> MGFVRQIQLLLWKNWTLRKRQKIRFVVELVWPLSLFLVLIWLRNANPLYSHHECHFPNKAMPSAGMLPWLQGIFCNVNNPCFQSPTPGESPGIVSNYNNSILARVYRDFQELLMNAPESQHLGRIWTELHILSQFMDTLRTHPERIAGRGIRIRDILKDEETLTLFLIKNIGLSDSVVYLLINSQVRPEQFAHGVPDLALKDIACSEALLERFIIFSQRRGAKTVRYALCSLSQGTLQWIEDTLYANVDFFKLFRVLPTLLDSRSQGINLRSWGGILSDMSPRIQEFIHRPSMQDLLWVTRPLMQNGGPETFTKLMGILSDLLCGYPEGGGSRVLSFNWYEDNNYKAFLGIDSTRKDPIYSYDRRTTSFCNALIQSLESNPLTKIAWRAAKPLLMGKILYTPDSPAARRILKNANSTFEELEHVRKLVKAWEEVGPQIWYFFDNSTQMNMIRDTLGNPTVKDFLNRQLGEEGITAEAILNFLYKGPRESQADDMANFDWRDIFNITDRTLRLVNQYLECLVLDKFESYNDETQLTQRALSLLEENMFWAGVVFPDMYPWTSSLPPHVKYKIRMDIDVVEKTNKIKDRYWDSGPRADPVEDFRYIWGGFAYLQDMVEQGITRSQVQAEAPVGIYLQQMPYPCFVDDSFMIILNRCFPIFMVLAWIYSVSMTVKSIVLEKELRLKETLKNQGVSNAVIWCTWFLDSFSIMSMSIFLLTIFIMHGRILHYSDPFILFLFLLAFSTATIMLCFLLSTFFSKASLAAACSGVIYFTLYLPHILCFAWQDRMTAELKKAVSLLSPVAFGFGTEYLVRFEEQGLGLQWSNIGNSPTEGDEFSFLLSMQMMLLDAAVYGLLAWYLDQVFPGDYGTPLPWYFLLQESYWLGGEGCSTREERALEKTEPLTEETEDPEHPEGIHDSFFEREHPGWVPGVCVKNLVKIFEPCGRPAVDRLNITFYENQITAFLGHNGAGKTTTLSILTGLLPPTSGTVLVGGRDIETSLDAVRQSLGMCPQHNILFHHLTVAEHMLFYAQLKGKSQEEAQLEMEAMLEDTGLHHKRNEEAQDLSGGMQRKLSVAIAFVGDAKVVILDEPTSGVDPYSRRSIWDLLLKYRSGRTIIMSTHHMDEADLLGDRIAIIAQGRLYCSGTPLFLKNCFGTGLYLTLVRKMKNIQSQRKGSEGTCSCSSKGFSTTCPAHVDDLTPEQVLDGDVNELMDVVLHHVPEAKLVECIGQELIFLLPNKNFKHRAYASLFRELEETLADLGLSSFGISDTPLEEIFLKVTEDSDSGPLFAGGAQQKRENVNPRHPCLGPREKAGQTPQDSNVCSPGAPAAHPEGQPPPEPECPGPQLNTGTQLVLQHVQALLVKRFQHTIRSHKDFLAQIVLPATFVFLALMLSIVIPPFGEYPALTLHPWIYGQQYTFFSMDEPGSEQFTVLADVLLNKPGFGNRCLKEGWLPEYPCGNSTPWKTPSVSPNITQLFQKQKWTQVNPSPSCRCSTREKLTMLPECPEGAGGLPPPQRTQRSTEILQDLTDRNISDFLVKTYPALIRSSLKSKFWVNEQRYGGISIGGKLPVVPITGEALVGFLSDLGRIMNVSGGPITREASKEIPDFLKHLETEDNIKVWFNNKGWHALVSFLNVAHNAILRASLPKDRSPEEYGITVISQPLNLTKEQLSEITVLTTSVDAVVAICVIFSMSFVPASFVLYLIQERVNKSKHLQFISGVSPTTYWVTNFLWDIMNYSVSAGLVVGIFIGFQKKAYTSPENLPALVALLLLYGWAVIPMMYPASFLFDVPSTAYVALSCANLFIGINSSAITFILELFENNRTLLRFNAVLRKLLIVFPHFCLGRGLIDLALSQAVTDVYARFGEEHSANPFHWDLIGKNLFAMVVEGVVYFLLTLLVQRHFFLSQWIAEPTKEPIVDEDDDVAEERQRIITGGNKTDILRLHELTKIYPGTSSPAVDRLCVGVRPGECFGLLGVNGAGKTTTFKMLTGDTTVTSGDATVAGKSILTNISEVHQNMGYCPQFDAIDELLTGREHLYLYARLRGVPAEEIEKVANWSIKSLGLTVYADCLAGTYSGGNKRKLSTAIALIGCPPLVLLDEPTTGMDPQARRMLWNVIVSIIREGRAVVLTSHSMEECEALCTRLAIMVKGAFRCMGTIQHLKSKFGDGYIVTMKIKSPKDDLLPDLNPVEQFFQGNFPGSVQRERHYNMLQFQVSSSSLARIFQLLLSHKDSLLIEEYSVTQTTLDQVFVNFAKQQTESHDLPLHPRAAGASRQAQD

ABCA4 is an ATP-binding cassette (ABC) transporter that flips N-retinylidene-phosphatidylethanolamine (N-Ret-PE) from the lumen to the cytoplasmic leaflet of photoreceptor membranes. Human ABCA4 is a 2273 amino acid full transporter organized in two nonidentical tandem halves with each half containing a transmembrane domain (TMD) consisting of six membrane-spanning segments, a nucleotide-binding domain (NBD), and a large glycosylated exocytoplasmic domain (ECD) between the first and second membrane-spanning segments. Unlike other ABCA transporters and other characterized eukaryotic ABC transporters that function as exporters, ABCA4 is an importer translocating either the all-trans or 11-cis isomers of N-Ret-PE from the lumen to the cytoplasmic leaflet of disc membranes. The importance of this transport activity is evident by the finding that over 1200 mutations in the gene encoding ABCA4 are known to cause Stargardt disease (STGD1), an autosomal recessive macular degenerative disease characterized by severe loss in central vision, degeneration of photoreceptors and underlying retinal pigment epithelial cells, and the accumulation of lipofuscin deposits containing di-retinoid compounds.

The cryo-EM map of substrate-free ABCA4 produced a final reconstruction with an overall “gold standard” resolution of 3.6 Å. ABCA4 exhibits a highly elongated shape with a length of 230 Å, a width of 85 Å, and domain organization as previously reported for other ABCA transporters. TMD1 and TMD2, each consisting of six transmembrane segments (TM), display an outward-facing conformation as found for ABCA1. Density corresponding to a lipid is lodged between TM1/2/11 at the level of the cytoplasmic leaflet of the membrane. This feature, also found in the ABCA1 structure, most likely represents a structural lipid important for stabilizing the protein. An elongated tunnel or cavity accessible to the intradiscal space and lined with hydrophobic residues is found extending through the central and lid regions. In our structure, we resolved five disulfide bonds, three within ECD1 (C54-C81, C75-C324, C370-C519), one in ECD2 (C1488-C1502) and one connecting ECD1 with ECD2 (C641-C1490) as inferred from an earlier biochemical study. Eight asparagine residues post-translationally modified with N-linked glycosylation are evident with four in ECD1 (N98, N415, N444, N504) and four in ECD2 (N1469, N1529, N1588, N1662) in agreement with earlier biochemical techniques. As observed in Type V ABC transporters, the NBDs are closely positioned opposite each other in a head-to-tail configuration. The substrate-free structure determined here is highly similar to that described in this recent study although different detergents were employed in the purification of the protein.3-(4-fluoranylphenoxy)-1-thiomorpholin-4-yl-propan-1-one 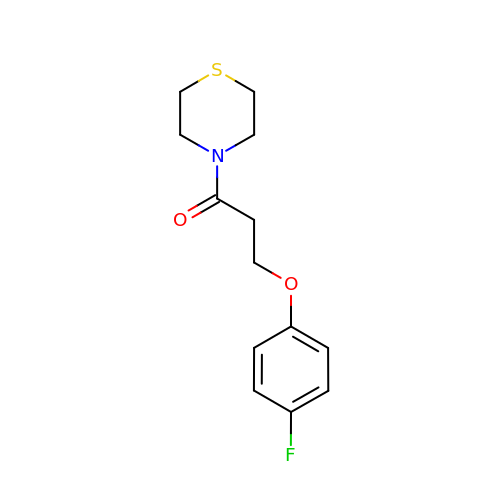| C13 H16 F N O2 S | WKRDDFLIYSQAFI-UHFFFAOYSA-N> ADFDYVVVGAGNAGNVVAARLTEDPDVSVLVLEAGVSDENVLGAEAPLLAPGLVPNSIFDWNYTTTAQAGYNGRSIAYPRGRMLGGSSSVHYMVMMRGSTEDFDRYAAVTGDEGWNWDNIQQFVRKNEMVVPPADNHNTSGEFIPAVHGTNGSVSISLPGFPTPLDDRVLATTQEQSEEFFFNPDMGTGHPLGISWSIASVGNGQRSSSSTAYLRPAQSRPNLSVLINAQVTKLVNSGTTNGLPAFRCVEYAEQEGAPTTTVCAKKEVVLSAGSVGTPILLQLSGIG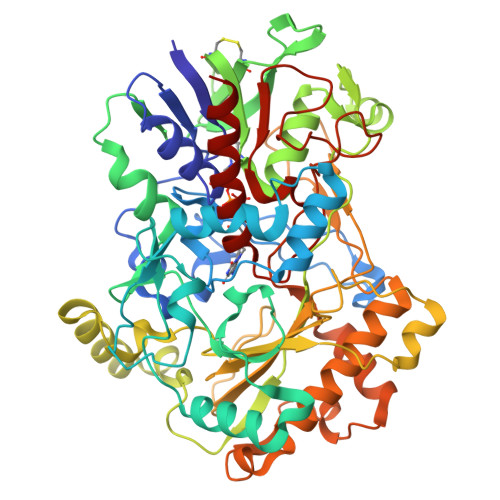DENDLSSVGIDTIVNNPSVGRNLSDHLLLPAAFFVNSNQTFDNIFRDSSEFNVDLDQWTNTRTGPLTALIANHLAWLRLPSNSSIFQTFPDPAAGPNSAHWETIFSNQWFHPAIPRPDTGSFMSVTNALISPVARGDIKLATSNPFDKPLINPQYLSTEFDIFTMIQAVKSNLRFLSGQAWADFVIRPFDPRLRDPTDDAAIESYIRDNANTIFHPVGTASMSPRGASWGVVDPDLKVKGVDGLRIVDGSILPFAPNAHTQGPIYLVGKQGADLIKADQ In Streptomyces scabiei, the causative agent of common scab in root and tuber crops, a genetic compensation phenomenon safeguards the loss of the gene encoding the cello-oligosaccharide hydrolase BglC by awakening the expression of alternative beta-glucosidases. Here, we revealed that the BglC compensating enzyme BcpE2 was the GH3-family beta-glucosidase that displayed the highest reported substrate promiscuity and was able to release the glucose moiety of all tested types of plant-derived heterosides (aryl β-glucosides, monolignol glucosides, cyanogenic glucosides, anthocyanosides, and coumarin heterosides). The exceptional substrate promiscuity of BcpE2 provides microorganisms a versatile tool for scavenging glucose from plant-derived nutrients that widely vary in size and structure. In this work, we reported the structural and biochemical characterization of BcpE2, a GH3-family β-glucosidase of the common scab phytopathogen S. scabiei.

We obtained the crystallographic structure of BcpE2 at 3.09 Å. The crystal belongs to the P3121 space group with one molecule in the asymmetric unit. Six regions could not be built because of a lack of electron density: the first nine amino acids (AA), the 12 C-terminal residues, which consist of a His6-Tag and a linker, and four loops (residues 70 to 73, 336 to 339, 436 to 443 and 531 to 536). BcpE2 is monomeric and is made of four domains: an N-terminal (β/α)8 TIM barrel domain (residues 10 to 306), an (α/β)6-sandwich domain (residues 316 to 398 and 551 to 650), a PA14 domain (residues 404 to 548), and a C-terminal fibronectin type III-like (fn3) domain (residues 711 to 821). In addition, a 60 AA linker is present between (α/β)6-sandwich and the fibronectin type III-like domains and mostly runs on the (β/α)8 TIM barrel domain. The two catalytic residues – Asp239 and Glu582 – were strictly conserved in all homologous GH3s. The active site of BcpE2 also included Asp59, Arg127, and three additional aromatic AAs, namely, Tyr207, Trp240, and Phe499, which were generally conserved in the closest GH3-family enzymes. The PA14 domain of BcpE2 was also characterized by B factor values significantly higher than the rest of the protein, particularly in the active site vicinity, indicating the likely flexibility of this domain. In BcpE2, Phe499 was equivalent when the two PA14 domains were superimposed independently (Cα 2 Å apart) but was shifted toward the position that the substrate would likely occupy when the entire structures were superimposed (Cα 5 Å apart). The BcpE2 structure revealed two features likely contributing to its broad substrate specificity, i.e., (i) a wide cavity in the PA14 domain connected to the d-glucose specific subsite (−1), and (ii) the high flexibility of this domain, especially the structure elements defining this cavity.

> MAATPGTRTTPADEAREAAVEKALAALDLDAKARLLSGQDMWTLPALPEIGLASLVMSDGPIGVRGVRWTADDPSVALPSPTALAATWDPGLARRAGVLLAQEARRKGVHVLLAPTVNLHRSPLGGRHFEAYSEDPYLTGEIGSGYVTGVQAGGVGTTVKHFVANDAETDRFTVNNLVSARALRELYLAPFEAIVANAHPWGIMTAYNQVNGSTMTEHRYLVNEVLRGEWGFDGFNVSDWLAARSTTGALTGGLDVAMPGPATVYGEPLAAAVRAGEVTESLLDEAVRRVLRLAARVGILEGAAPAVTELPAPVDGEALAREIARRSFVLVRNEVRDGRAALPLEQGATVALIGAAARDARVLGGGSATVFPARVVSPLDGLTAALPEGAPTYALGADPNEELAVADTGFTLRAVCRDASGTVIGTRSAPNGHIQWMGSDLPDGVTHATLHSVELTGTFTPRETGTHTFGVKGLGAYTLTVDGTTHFDGVRTTDTDDPFVSFFGAPVPLAEVELTEGTPLEVSLTHVVELAADAPITMLAFSLCHQEPQRDPDELIAEAVEAARAADTAVVVVATTERVESEGFDRKDLRLPGRQDDLVRAVAAANPATVVVVNAGSPVELPWREDVAAVLLTWFPGQEGGAALAEVLTGAHEPGGRLPTTWGSLTGAPVTQVTPTAGELVYDEGVFIGYRAWDKEDRTPTYPFGHGLGYTDWTYESLDVTGTTATVRVRNTGTREGRETVQLYLAPTTADENRPTRWLAGFATVEAAPGETAEAVVRLPRRAFEIWDETTGAWVYVTGSYEVAAGRSIADRRTRVTIEAPKLAAALEHHHHHH> MLRSSLRYGVHKVGYTHPHHLPVPCAQRWDLRL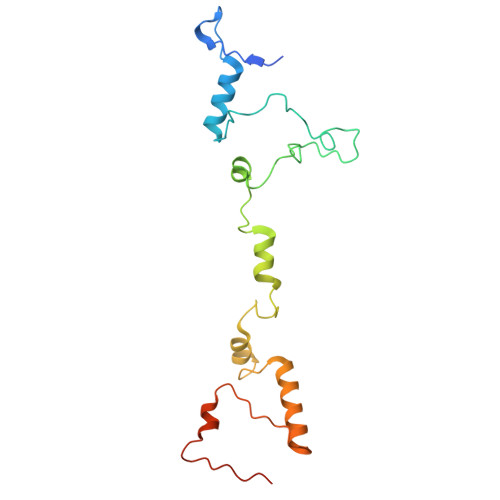ARARIFQEYIEEKAPGAWQLEDERHMSPEFNTFTGYPMRNLRPGYGQNLPEFIMKKRLPNNTHYELFARRDIPNEDNAMYGKLLYDMTIHGTSLPSIYRMHKDINKAQRNDRKLSGNRFKVLNSSGAKSPPSGFEAIPDAVEEEDD> GPLGSDHDDSFHVILNKS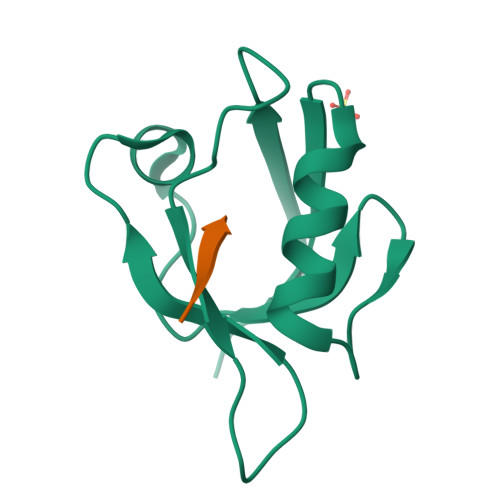SPEEQLGIKLVRRVDEPGVFIFNVLNGGVADRHGQLEENDRVLAINGHDLRFGSPESAAHLIQASERRVHLVVSRQ;> YKVRNVTLV> ADQPIDADVTVIGSGPGGYVAAIKAAQLGFKTVCIEKNETLGGTCLNVGCIPSKALLNNSHYYHMAHGTDFASRGIEMSEVRLNLDKMMEQKSTAVKALTGGIAHLFKQNKVVHVNGYGKITGKNQVTATKADGGTQVIDTKNILIATGSEVTPFPGITIDEDTIVSSTGALSLKKVPEKMVVIGAGVIGVELGSVWQRLGADVTAVEFLGHVGGVGIDMEISKNFQRILQKQGFKFKLNTKVTGA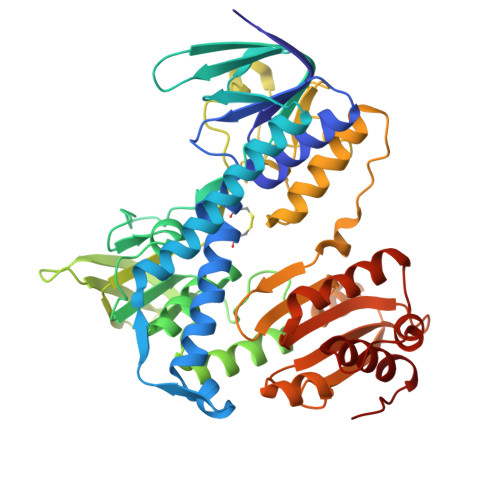TKKSDGKIDVSIEAASGGKAEVITCDVLLVCIGRRPFTKNLGLEELGIELDPRGRIPVNTRFQTKIPNIYAIGDVVAGPMLAHKAEDEGIICVEGMAGGAVHIDYNCVPSVIYTHPEVAWVGKSEEQLKEEGIEYKVGKFPFAANSRAKTNADTDGMVKILGQKSTDRVLGAHILGPGAGEMVNEAALALEYGASCEDIARVCHAHPTLSEAFREANLAASFGKSINF> GAMDTFVQHIKRHNIVLKRELGEGAFGKV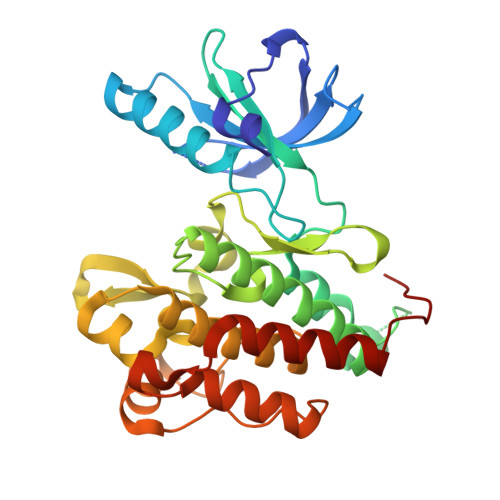FLAECYNLCPEQDKILVAVKTLKDASDNARKDFHREAELLTNLQHEHIVKFYGVCVEGDPLIMVFEYMKHGDLNKFLRAHGPDAVLMAEGNPPTELTQSQMLHIAQQIAAGMVYLASQHFVHRDLATRNCLVGENLLVKIGDFGMSRDVYSTDYYRVGGHTMLPIRWMPPESIMYRKFTTESDVWSLGVVLWEIFTYGKQPWYQLSNNEVIECITQGRVLQRPRTCPQEVYELMLGCWQREPHMRKNIKGIHTLLQNLAKASPVYLDILG> SNAMSINTTLLTPELYQYLLQVSLREPPLLAELREETTRSFSTYAMQTAPEQAQLLALLVKLMQAKKVIDIGTFTGYSAIAMGLALPKDGTLITCDVDEKSTALAKEYWEKAGLSDKIGLRLSPAKDTLAELIHAGQAWQYDLIY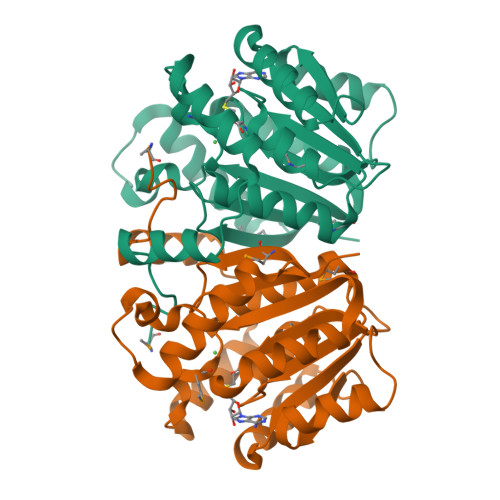IDADKANTDLYYEESLKLLREGGLIAVDNVLRRGQVADEENQSENNQLIRLFNQKVYKDERVDMILIPIGDGLTLARKKS>MDNKITDEQIAEWNSKQEELRDKIIRSDGDFSLSKVKYVGGFDVSYSKINHELAVSCMVVLSYPEMKQVYMNTTKVKLSCPYKSSYLAFREIEPFQQELQLLKAKKPNLEPQVFLLDGNGFFHIRRCGAASHLGVLSNTRTIGVAKSLIEIPEDGVKKTEVISQFKRLRKTGGNELDIISTEKNEVLAKAVLYAPKVEKPIFVSAGHKCSLETAAKIVKGCTKTRIPEPIKMADKWSRKELKKIE[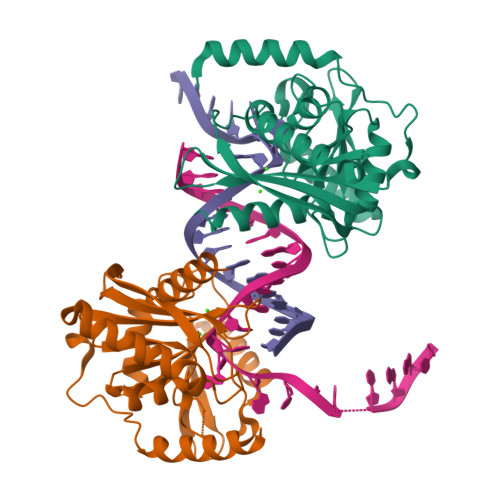4x]>CTSLTLETADRKHVLARTMDFAFQLGTEVILYPRRYSWNSEADGRAHQTQYAFIGMGRKLGNILFADGINESGLSCAALYFPGYAEYEKTIREDTVHIVPHEFVTWVLSVCQSLEDVKEKIRSLTIVEKKLDLLDTVLPLHWILSDRTGRNLTIEPRADGLKVYDNQPGVMTNSPDFIWHVTNLQQYTGIRPKQLESKEMGGLALSAFGQG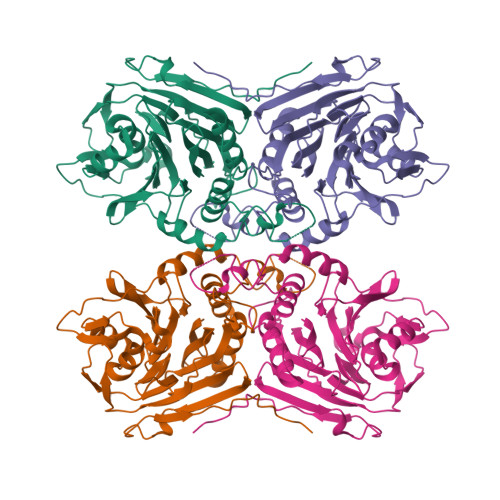LGTVGLPGDYTPPSRFVRAVYLKEHLEPAADETKGVTAAFQILANMTIPKGAVITEEDEIHYTQYTSVMCNETGNYYFHHYDNRQIQKVNLFHEDLDCLEPKVFSAKAEESIHELN[2x]>MSDRFVIWAPSMHNEPAAKCGYCHGNKGGNMDQLFALDSWAHRYMNKMDVVKIENCTIGSFVEHMDVATYDRMCNMGFRRSGKFLYKVDPLRNCCRLYTIRTAPQELNMTKELKKCISRFATRITSEDYCPAAVASSDFVGKIVNAEMNSKTFYTRFEPALYSEEKYHLFVKYQEKVHQDYNNSPKSFKRFLCDTPFGPEAVLGTQESWEQLNNWQRMKPGEKLKHMGPVHECYYYEGKLIAITVSDILPSGISSVYFIWDPDYSKWSLGKLSALRDLAIIQRTNLQYYYLG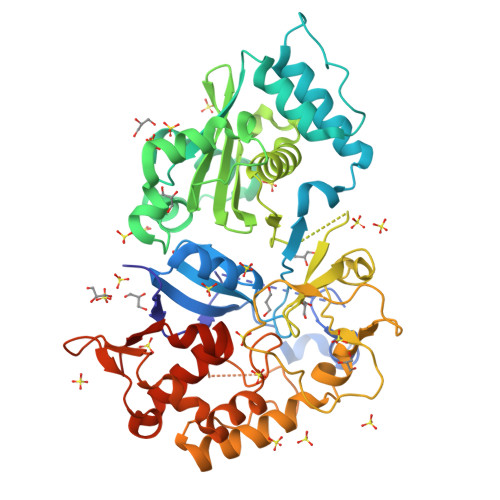YYIEDCPKMNYKANYGAEVLDVCHSKYIPLKPIQDMISRGKLFVIGEEETKVTKELYLVDSETGRGEGFPTDNVVKYKNIAEEIYGVGGCAFKSANESALELKELYGIPYEEEDLDTIYHLKEHNGHAPNGIPNVVPGLLPLWELLDIMQSGKITDLEGRLFLFEIETEGIRPLINFYSEPPNVKKRICDVIRLFGFETCMKAVILYSEQMENLYFQSLEHHHHHH[12x]>GAMDPEFMNKYQAVIIGFGKAGKTLAVTLAKAGWRVALIEQSNAMYGGTCINIGCIPTKTLVHDAQQHTDFVRAIQRKNEVVNFLRNKNFHNLADMPNIDVIDGQAEFINNHSLRVHRPEGNLEIHGEKIFINTGAQTVVPPIPGITTTPGVYDSTGLLNLKELPGHLGILGGGYIGVEFASMFANFGSKVTILEAASLFLPREDRDIADNIATILRDQGVDIILNAHVERISHHENQVQVHSEHAQLAVDALLIASGRQPATASLHPENAGIAVNERGATVVDKRLHTTADNIWAMGDVTGGLQFTYISLDDYRIVRDELLGEGKRSTDDRKNVPYSVFMTPPLSRVGMTEEQARESGADIQVVTLPVAAIPRARVMNDTRGVLKAIVDNKTQRMLGASLLCVDSHEMINIVKMVMDAGLPYSILRDQIFTH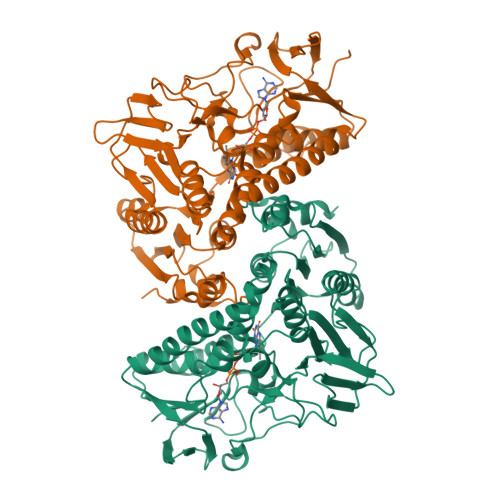PSMSESLNDLFSLVK[4x]> GSFTMDLVEEILRLKEERNAIILAHNYQLPEVQDIADFIGDSLELARRATRVDADVIVFAGVDFMAETAKILNPDKVVLIPSREATCAMANMLKVEHILEAKRKYPNAPVVLYVNSTAEAKAYADVTVTSANAVEVVKKLDSDVVIFGPDKNLAHYVAKMTGKKIIPVPSKGHCYVHQKFTLDDVERAKKLHPNAKLMIHPECIPEVQEKADIIASTGGMIKRACEWDEWVVFTEREMVYRLRKLYPQKK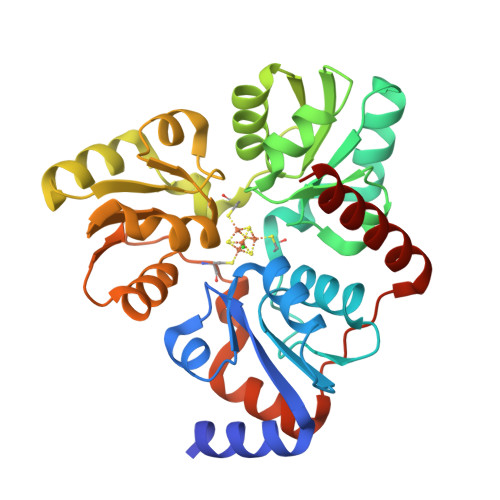FYPAREDAFCIGMKAITLKNIYESLKDMKYKVEVPEEIARKARKAIERMLEMSK>[2x]MFENITAAPADPILGLADLFRADERPGKINLGIGVYKDETGKTPVLTSVKKA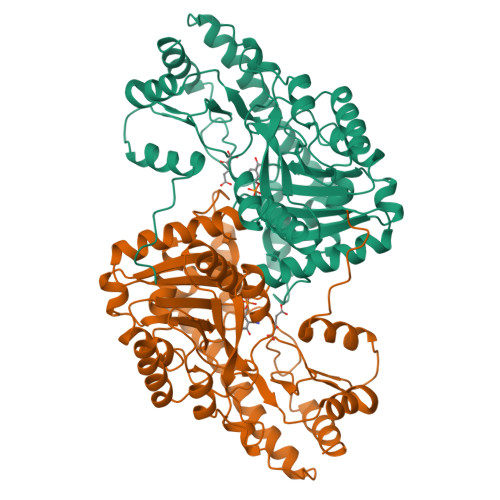EQYLLENETTKNYLGIDGIPEFGRCTQELLFGKGSALINDKRARTAQTPGGTGALRVAADFLAKNTSVKRVWVSNPSWPNHKSVFNSAGLEVREYAYYDAENHTLDFDALINSLNEAQAGDVVLFHGCCHNPTGIDPTLEQWQTLAQLSVEKGWLPLFDFAYQGFARGLEEDAEGLRAFAAMHKELIVASSYSHNFGLYNERVGACTLVAADSETVDRAFSQMKAAIRANYSNPPAHGASVVATILSNDALRAIWEQELTDMRQRIQRMRQLFVNTLQEKGANRDFSFIIKQNGMFSFSGLTKEQVLRLREEFGVYAVASGRVNVAGMTPDNMAPLCEAIVAVL>MADETIAIVDADATAETRSLLSYLDGVRGEGILFGHQHTTSFGLTTGPTDGTTSDVKNVTGDFPAVFGWDTLIIEGNERPGLAENTRDENIALFADYIRKADAIGGVNTVSAHVENFVTGGSFYDTSGDTLRAVLPGGSHHAELVAYLDDIAELADASRRDDGTLIPIVFRPWHENAGSWFWWGAAYGSPGEYQELYRFTVEYLRDVKGVSNFLYAWGPGGGFGGNRDVYLRTYPGDAFVDVLGLDTYDSTGSDAFLAGLVA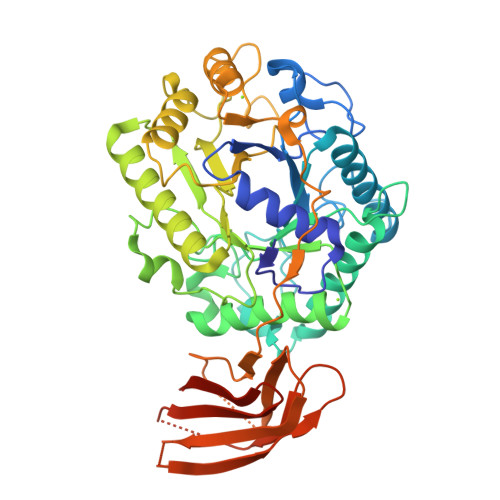DLRMIAEIADEKGKVSAFTEFGVSGGVGTNGSSPAQWFTKVLAAIKADPVASRNAYMETWRNADAGQHFVPVPGDALLEDFQAYAADPFTLFASEVTGAFDRTVAAAPAQPVVHIASPADGARVASAPTTVRVRVGGTDVQSVTVEVAQGGTVVDTLDLAYDGALWWTAPWSPTSAQLDNSTYTVTATATTAAGTLDVTNEVAAALEHHHHHH[2x]>TESEKSLMSRTGGLGAPRGQAFWPVRGPTLHRYGEQLQGELRWKGMVIGASEGTEVKAIADGRVILADWLQGYGLVVVVEHGKGDMSLYGYNQSALVSVGSQVRAGQPIALVGSSGGQGRPSLYFEIRRQGQAVNPQPWLG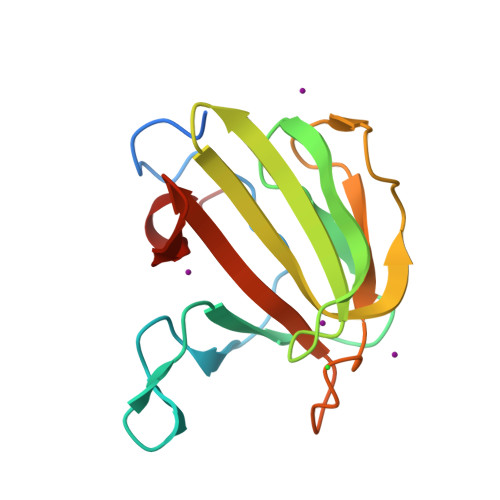R[4x]>[2x]GNYKKPKLLYCSNGGHFLRILPDGTVDGTRDRSDQHIQLQLSAESVGEVYIKSTETGQYLAMDTDGLLYGSQTPNEECLFL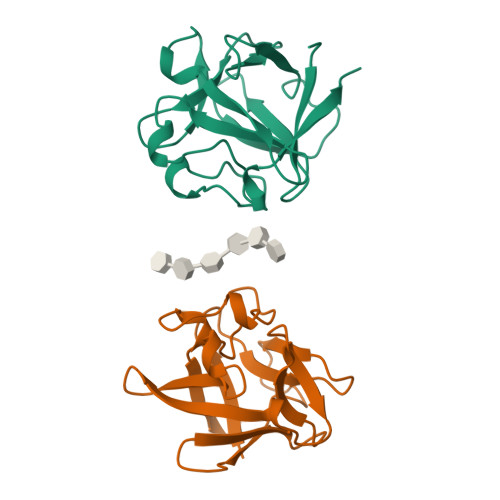ERLEENHYNTYISKKHAEKNWFVGLKKNGSCKRGPRTHYGQKAILFLPLPVSSD>MNSSLPSLRDVFANDFRIGAAVNPVTIEMQKQLLIDHVNSITAENHMKFEHLQPEEGKFTFQEADRIVDFACSHRMAVRGHTLVWHNQTPDWVFQDGQGHFVSRDVLLERMKCHISTVVRRYKGKIYCWDVINEAVADEGNELLRPSKWRQIIGDDFMEQAFLYAYEADPDALLFYNDYNECFPEKREKIFALVKSLRDKGIPIHGIGMQAHWSLTRPSLDEIRAAIERYASLGVVLHITGLDVSMFEFHDRRTDLAAPTSEMIERQAERYGQIFALFKEYRDVIQSVTFWGIADDH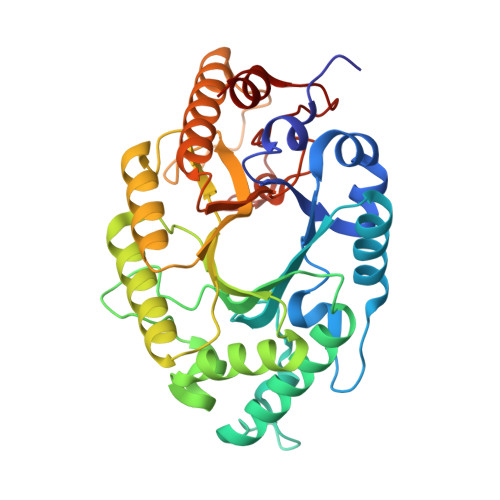TWLDNFPVHGRKNWPLLFDEQHKPKPAFWRAVSV[2x]> MQWSGARALEALLTVAGELRGPPLQLDTGQL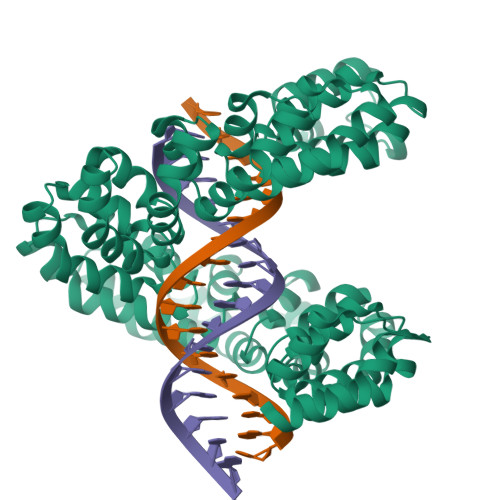LKIAKRGGVTAVEAVHAWRNALTGAPLNLTPEQVVAIASHDGGKQALETVQRLLPVLCQAHGLTPQQVVAIASHDGGKQALETVQRLLPVLCQAHGLTPEQVVAIASHDGGKQALETVQALLPVLCQAHGLTPEQVVAIASNGGGKQALETVQRLLPVLCQAHGLTPQQVVAIASNGGGKQALETVQRLLPVLCQAHGLTPQQVVAIASNGGGKQALETVQRLLPVLCQAHGLTPQQVVAIASNIGGKQALETVQRLLPVLCQAHGLTPQQVVAIASNGGGKQALETVQRLLPVLCQAHGLTPQQVVAIASHDGGKQALETVQRLLPVLCQAHGLTPEQVVAIASNGGGKQALETVQRLLPVLCQAHGLTPEQVVAIASHDGGKQALETVQRLLPVLCQAHGLTPQQVVAIASNGGGRPALESIVAQLSRPDPALAALTNDHLVALACLGGRPALDAVKKLEHHHHHH N-(morpholin-4-ylcarbonyl)-L-phenylalanyl-N-[(1R,2S)-1-(cyclohexylmethyl)-2-hydroxy-3-(1-methylethoxy)-3-oxopropyl]-S-methyl-L-cysteinamide 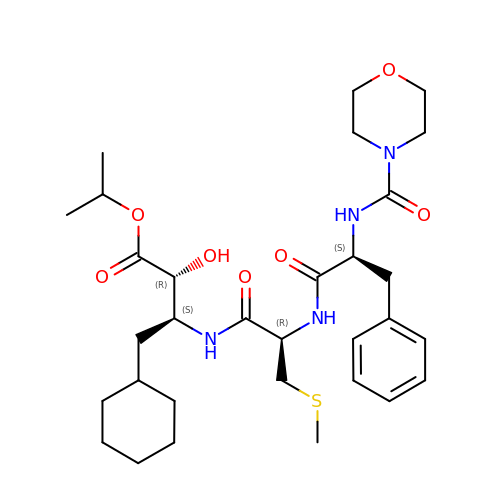| C31 H48 N4 O7 S | UZQBKCWYZBHBOW-YIPNQBBMSA-N COENZYME 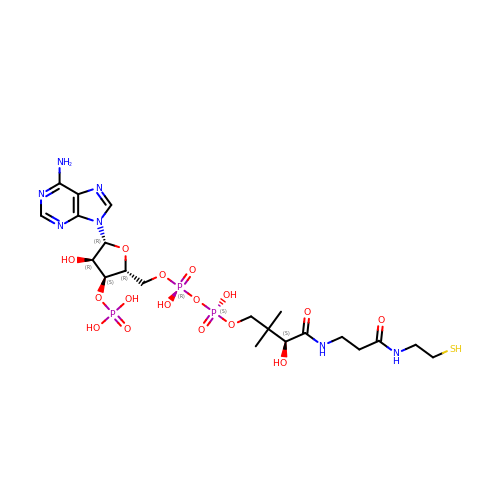A | C21 H36 N7 O16 P3 S | RGJOEKWQDUBAIZ-HDCXRZRFSA-N> SGRPSTDALKLCPHEEFLRLCKERAEEIYPIKERNNRT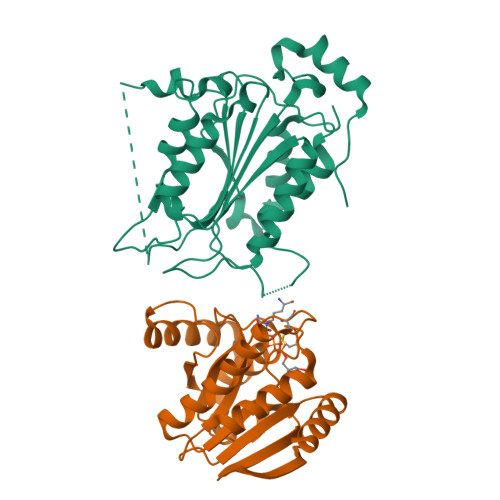RLALIICNTEFDHLPPRNGADFDITGMKELLEGLDYSVDVEENLTARDMESALRAFATRPEHKSSDSTFLVLMSHGILEGICGTVHDEKKPDVLLYDTIFQIFNNRNCLSLKDKPKVIIVQAARGANRGELWVRDSPASLEVASSQSSENLEEDAVYKTHVEKDFIAFCSSTPHNVSWRDSTMGSIFITQLITCFQKYSWCCHLEEVFRKVQQSFETPRAKAQMPTIERLSMTRYFYLFPGN;> GPLGSGRPMEVLFEAKVGDITLKLAQGDITQYPAKAIVNAANKRLEHGGGVAYAIAKACAGDAGLYTEISKKAMREQFGRDYIDHGEVVVTPAMNLEERGIKYVFHTVGPICSGMWSEELKEKLYKAFLGPLEKAEEMGVESIAFPAVSAGIYGCDLEKVVETFLEAVKNFKGSAVKEVALVIYDRKSAEVALKVFERSL>GCG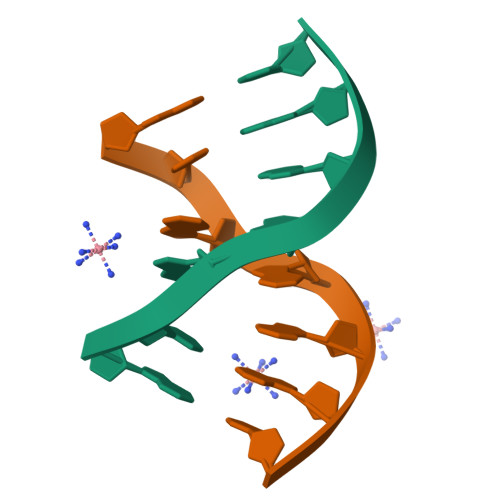AAGC[6x]>MGRGSHHHHHHGMAMNIKELSLHELCEELKTPAWNVPLTFVGDVGGTSARMGFVREGKNDSVHACVTRYSMKRKDITELIEFFN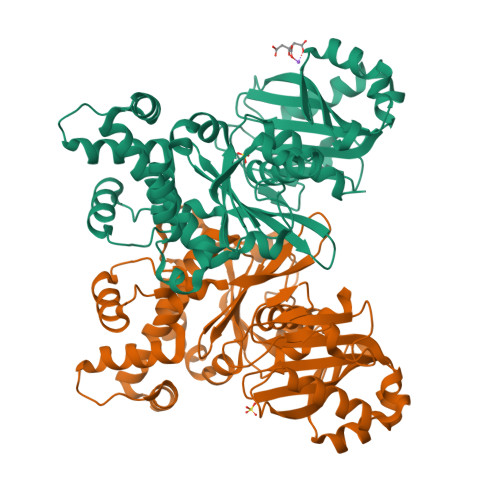EIIELMPASVIKRVKAGVINVPGPVTGGAVGGPFNNLKGIARLSDYPKALFPPGRSAILNDLEAGGFGVLAVSDAHVFSEYFGVMWEGTQWRTCEQEPAGSVIGRGRCLVLAPGTGLGSSLIYYNPMNQQHIVVPLELGSQTIPMRKDIDYIQTLHAELKLLPNYENMVSGAGLEFHYRQVVRGSRPPCSAGEIAKLASEGDANACKAMKKYHEYLMRVGSEASMALLPLTIVLVGDNIVNNAFFYRNPQNLKEMHREALNHEMERFGFQSRVTYLRQKKLLNLNLMGCYRCGLDLS[2x]> MRVNNGLTPQELEAYGI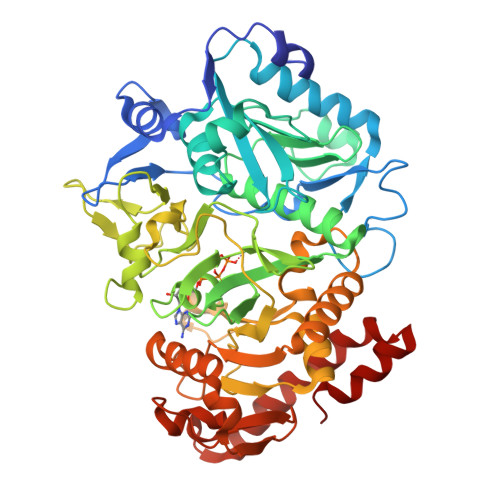SDVHDIVYNPSYDLLYQEELDPSLTGYERGVLTNLGAVAVDTGIFTGQSPKDKYIVRDDTTRDTFWWADKGKGKNDNKPLSPETWQHLKGLVTRQLSGKRLFVVDAFCGANPDTRLSVRFITEVAWQAHFVKNMFIRPSDEELAGFKPDFIVMNGAKCTNPQWKEQGLNSENFVAFNLTERMQLIGGTWYGGEMKKGMFSMMNYLLPLKGIASMHCSANVGEKGDVAVFFGLSGTGKTTLSTDPKRRLIGDDEHGWDDDGVFNFEGGCYAKTIKLSKEAEPEIYNAIRRDALLENVTVREDGTIDFDDGSKTENTRVSYPIYHIDNIVKPVSKAGHATKVIFLTADAFGVLPPVSRLTADQTQYHFLSGFTAKLAGTERGITEPTPTFSACFGAAFLSLHPTQYAEVLVKRMQAAGAQAYLVNTGWNGTGKRISIKDTRAIIDAILNGSLDNAETFTLPMFNLAIPTELPGVDTKILDPRNTYASPEQWQEKAETLAKLFIDNFDKYTDTPAGAALVAAGPKL>[2x]MPGLFLTLEGLDG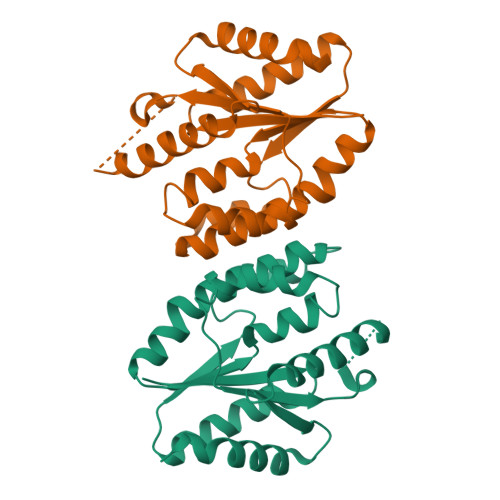SGMTTQARRLAAFLEAQGRPVLLTREPGGGLPEVRSLLLTQELSPEAEYLLFSADRAEHVRKVILPGLAAGKVVISDRYLDSSLAYQGYGRGLPLPWLREVAREATRGLKPRLTFLLDLPPEAALRRVRRPDRLEGLGLEFFRRVREGYLALARAEPGRFVVLDATLPEEEIARAIQAHLRPLLP Denitrification is the stepwise reduction of nitrogen oxides to dinitrogen and is utilized by many bacteria to replace the terminal oxygen-dependent steps of the respiratory chain under anaerobic conditions. The reduction of nitrite to nitric oxide is a highly regulated step, since both of these molecules are toxic to the cell. In NirS, these domains form homodimers by interaction of the 15th β-strand of each subunit, which is consistent with the SEC data collected during purification (data not shown). 1 nitrite reductase NirS adopts an open and a closed conformation, and it has been hypothesized that these states are linked to the catalytic cycle.

1-bound structures by a rotation of approximately 60° around the pseudo-eightfold axis of the β-propeller. A similar conformation has previously been observed for Pa-NirS after amino-acid exchange of His327 to alanine or for Pp-NirS crystallized under reducing conditions. 1-free NirS with other Pa-NirS structures reveals a higher similarity to the structure of NirS reduced in crystallo (Cα r.m.s.d. of 0.37 Å) compared with the oxidized form (Cα r.m.s.d. of 1.09 Å). The difference is mostly caused by the position of residues 55–64 and is consistent with an observation previously discussed for NirSH327A (Cα r.m.s.d. for cytochrome c of 0.35 Å). 1 domain reveals a lower Cα r.m.s.d. with respect to the H327A variant of Pa-NirS (0.75 Å) than to the oxidized or reduced wild-type protein (1.34 and 1.39 Å, respectively). Additionally, His327 and His369, which are both involved in substrate binding and catalysis by NirS, have different positions. Interestingly, the neighbouring loop (residues 473–479) also adopts a slightly different conformation. The open conformation of NirS may also have additional physiological importance outside the denitrification process. Therefore, the conformational change observed in our study can be envisioned to release the N-terminal arm to allow flagella formation, thereby regulating cell motility. Further investigation will be required to confirm that the conformational changes observed in crystallo can also be found in solution and are associated with distinct functions of NirS in vivo.

> KDDMKAAEQYQGAASAVDPAHVVRTNGAPDMSESEFNEAKQIYFQRCAGCHGVLRKGATGKPLTPDITQQRGQQYLEALITYGTPLGMPNWGSSGELSKEQITLMAKYIQHTPPQPPEWGMPEMRESWKVLVKPEDRPKKQLNDLDLPNLFSVTLRDAGQIALVDGDSKKIVKVIDTGYAVHISRMSASGRYLLVIGRDARIDMIDLWAKEPTKVAEIKIGIEARSVESSKFKGYEDRYTIAGAYWPPQFAIMDGETLEPKQIVSTRGMTVDTQTYHPEPRVAAIIASHEHPEFIVNVKETGKVLLVNYKDIDNLTVTSIGAAPFLHDGGWDSSHRYFMTAANNSNKVAVIDSKDRRLSALVDVGKTPHPGRGANFVHPKYGPVWSTSHLGDGSISLIGTDPKNHPQYAWKKVAELQGQGGGSLFIKTHPKSSHLYVDTTFNPDARISQSVAVFDLKNLDAKYQVLPIAEWADLGEGAKRVVQPEYNKRGDEVWFSVWNGKNDSSALVVVDDKTLKLKAVVKDPRLITPTGKFNVYNTQHDVY> MSNSDDEIQEIEAKRQKMSQEDSEVEIEILDEPEQGKLKNSSMSDEQKLHEFAIITATDEAFAQSILQDVDWDLKKALDVFYGSEAFAEARSAAVMGASSSMASSGAAVMTAEDLKGFEVSVMSWNIDGLDGRSLLTRMKAVAHIVKNVNPDILFLQEVVDRDLAPIDKLQSLYKIYYSNKGCQYYTAILVSKMFDVEKHDVIHFQNSGMYRTLQILEGSIGGLKVFLLNTHLESTREHRPQRCAQFGFCMDKVREIIAQNPGALVFFGGDLNL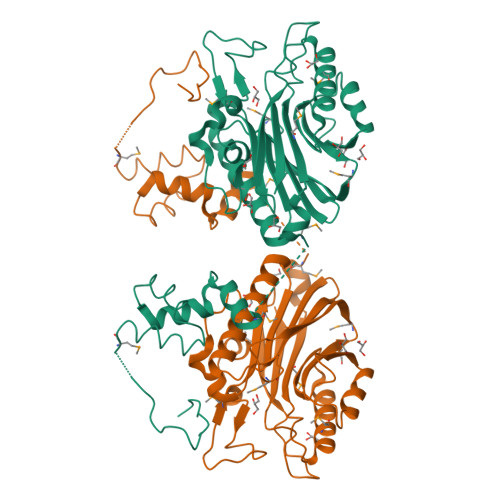RDEEVSRVPDGVKDAWEAAGSDNKTKFTWDTFKNDNKQGFHGAKMRFDRLYWSGPLDKVKFTLEGRQRIRSCLCFPSDHWAINATFFA>[2x]MENSLFNQEVQIPLTESYCGPCPKNWICYKNNCYQFFDESKNWYESQASCMSQNASLLKVYSKEDQDLLKLVKSYHWMGLVHIPTNGSWQWEDGSILSPNLLTIIEMQKGDCALYASSFKGYIENCSTPNTYICMQRTV;> MEPHSLR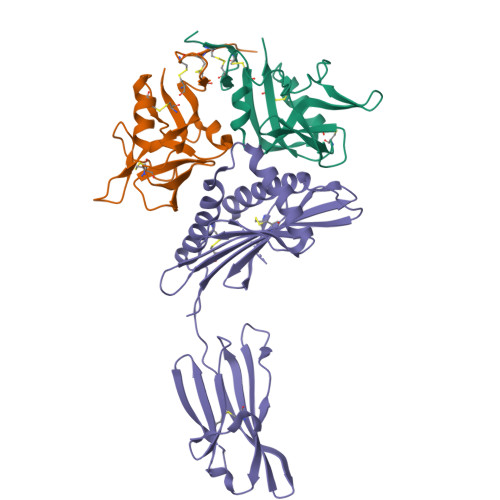YNLTVLIWDGSVQSGFLTEVHLDGQPFLRCDRQKCRAKPQGQWAEDVLGNKTWDRETRDLTGNGKDLRMTLAHIKDQKEGLHSLQEIRVCEIHEDNSTRSSIHFYYDGELFLSNNLETKEWTMPQSSRAQTLAMNVRNFWKEDAMKTKTHWHAMHADCLQELRRYLKSGVVLRRTVPPMVNVTRSEASEGNITVTCRASGFYPWNITLSWRQDGVSLSHDTQQWGDVLPDGNGTYQTWVATRICQGEEQRFTCYMEHSGNHSTHPVPS A major role in counteracting this equilibration to endomembranes is played by the guanine nucleotide dissociation inhibitor (GDI)-like solubilization factor PDEδ891011. It sequesters KRas from the cytosol by binding the farnesyl moiety, preventing that KRas binds to endomembranes and thereby enhancing its diffusion throughout the cell. Besides KRas, the PDEδ/Arl2 system is also crucial for maintaining membrane localization of other proteins of the Ras family, such as palmitoylated H- and N-Ras, as well as localization of the solely farnesylated Rheb on perinuclear membranes. Reducing PM localization of Ras through PDEδ inhibition raises alternative opportunities to impede oncogenic Ras signalling.

Herein, we describe the discovery of pyrazolopyridazinones as a novel PDEδ inhibitor chemotype that targets the prenyl-binding pocket of PDEδ with low nanomolar affinity. To identify alternative chemotypes for the inhibition of the PDEδ/Ras interaction with potency similar to Deltarasin (KD=38±16 nM), an in-house library of ∼150,000 compounds, assembled considering structural diversity of the underlying scaffolds, drug-likeness, coverage of different established drug target classes and inspiration by natural products, was subjected to high-throughput screening by means of the previously developed AlphaScreen Technology13. The screen revealed pyrazolopyridazinone 2a (KD=5±2 nM) as ligand of the prenyl-binding pocket of PDEδ. Structure-based development of the pyrazolopyridazinone hit class was enabled by a crystal structure of inhibitor 2a in complex with PDEδ at a resolution of 2.6 Å which revealed that, like inhibitors of the Deltarasin-type, heterocycle 2a employs H-bonds to Tyr 149 and Arg 61 for binding to PDEδ13. Initial screening and molecular modelling investigations (Schrödinger, Maestro suite) revealed that a C-3 linker between the two hydrogen-bonding groups is important and that shortening of the linker would abrogate H-bond formation between the amide carbonyl and Tyr 149. Therefore, a C-3 linker was kept for further inhibitor development. Since anilides display low metabolic stability, we searched for an alternative to the anilide embodied in hit compound 2a. Initial investigations and modelling revealed benzyl- and homobenzylamides as potential inhibitors, since they could adopt a conformation in which an H-bond with Tyr 149 is formed and the empty space in the PDEδ pocket is filled. Based on the fact that pyrazolopyridazinone 2a binds to PDEδ like the Deltarasin-type inhibitors, molecular modelling experiments indicated that 2k will form the same hydrogen bonds as Deltarasin and may additionally form a hydrogen bond with glutamine 78. Herein, we compared the newly developed PDEδ inhibitor Deltazinone 1 based on the pyrazolopyridazinone scaffold to the benzimidazole-based Deltarasin and the genetic knockdown of PDEδ.

>SAKDERAREILRGFKLNWMNLRDAATGKILWQGTEDLSVPGVEHEARVPKKILKCKAVSRELNFSSTEQMEKFRLEQKVYFKGQCLEEWFFEFGFVIPNSTNTWQSLIEAAPESQMMPASVLTGNVIIETKFFDDDLLVSTSRVRLFYV[2x]>MRFVHVKNPYLDLMDEDILYHLDLGTKTHNLPAMFGDVKFVCVGGSPNRMKAFALFMHKELGFEEAEEDIKDICAGTDRYCMYKTGPVLAISHGMGIPSISIMLHELIKLLHHARCCDVTIIRIGTSGGIGIAPGTVVITDIAVDSFFKPRFEQ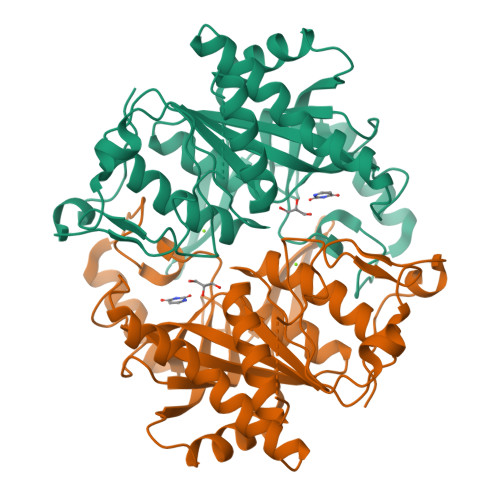VILDNIVTRSTELDKELSEELFNCSKEIPNFPTLVGHTMCTYDFYEGQGRLDGALCSFSREKKLDYLKRAFKAGVRNIEMESTVFAAMCGLCGLKAAVVCVTLLDRLDCDQINLPHDVLVEYQQRPQLLISNFIRRRLGLCDAHHHHHH[3x]>GSPCPGACVCYNEPKVTTSCPQQGLQAVPTGIPASSQRIFLHGNRISHVPAASFQSCRNLTILWLHSNALARIDAAAFTGLTLLEQLDLSDNAQLHVVDPTTFHGLGHLHTLHLDRCGLRELGPGLFRGLAALQYLYLQDNN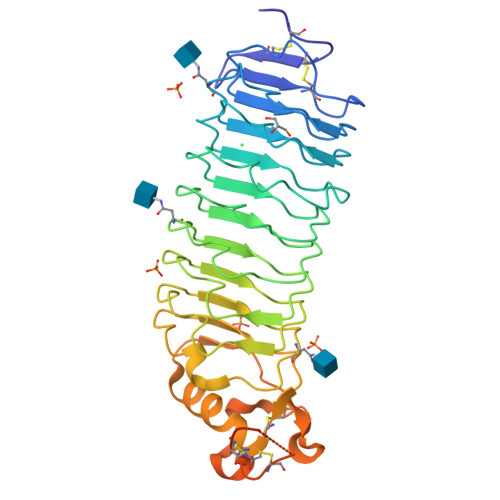LQALPDNTFRDLGNLTHLFLHGNRIPSVPEHAFRGLHSLDRLLLHQNHVARVHPHAFRDLGRLMTLYLFANNLSMLPAEVLMPLRSLQYLRLNDNPWVCDCRARPLWAWLQKFRGSSSEVPCNLPQRLADRDLKRLAASDLEGCAVASGPFRPIQTSQLTDEELLSLPKCCQPDAADKASVLEAAAHHHHHH[4x]>[2x]MLPGTFFEVLKNEGVVAI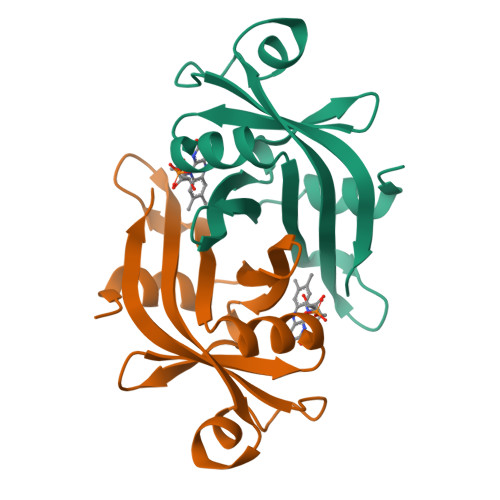ATQGEDGPHLVNTWDSYLKVLDGNRIVVPVGGMHKTEANVARDERVLMTLGSRKVAGRNGPGTGFLIRGSAAFRTDGPEFEAIARFKWARAALVITVVSAEQTL(R)-6-(3-amino-2-(5-(2-(6-amino-4-methylpyridin-2-yl)ethyl)pyridin-3-yl)propyl)-4-methylpyridin-2-amine 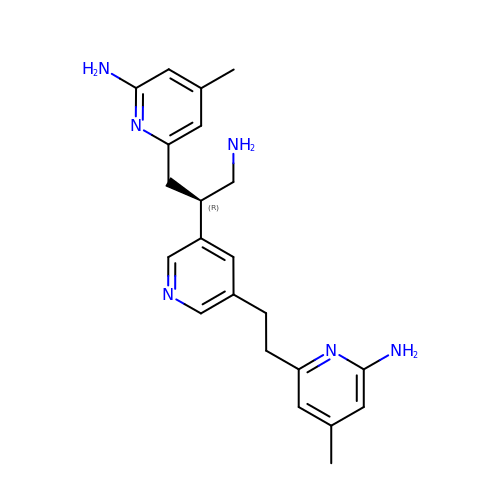| C22 H28 N6 | HKLFDCGBVFYQPQ-KRWDZBQOSA-N>[2x]MTKRIASVEKTIRIGFVGSLLFGLLPRIIHLYRQAHPNLRIELYEMGTKAQTEALKEGRIDAGFGRLKISDP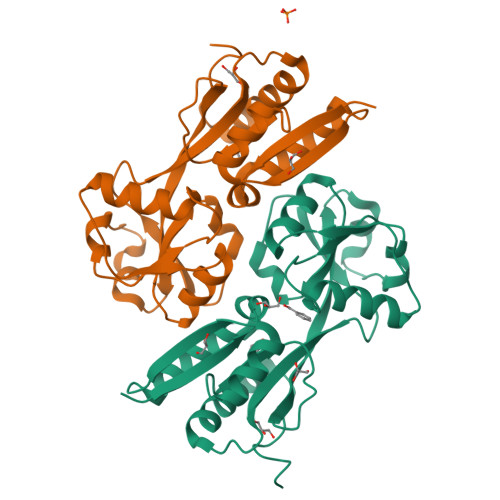AIKRTLLRNERLMVAVHASHPLNQMKDKGVHLNDLIDEKILLYPSSPKPNFSTHVMNIFSDHGLEPTKINEVREVQLALGLVAAGEGISLVPASTQSIQLFNLSYVPLLDPDAITPIYIAVRNMEESTYIYSLYETIRQIYAYEGFTEPPNWLEHHHHHH>MLENISSVKVSGGWHKQYTHSAVSTHCTMRFAVFLPPGASESNKVPVLYWLSGLTCTDENFMQKAGAFKKAAELGIAIVAPDTSPRGDNVPNEDSYDFAQGAGFYVNATQAPYNTHFNMYDYVVNELPALIEQHFPVTSTKAISGHSMGGHGALMI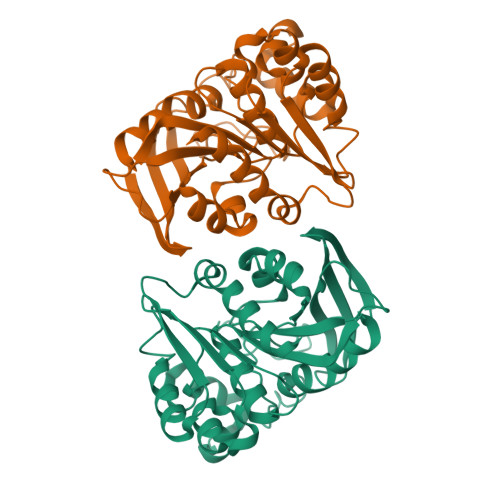ALKNPQDYVSASAFSPIVNPINCPWGVKAFTGYLGADKTTWAQYDSCKLMAKAEQSNYLPMLVSQGDADNFLDEQLKPQNLVAVAKQKDYPLTLEMQTGYDHSYFFISSFIDQHLVFHHQYLSA[4x]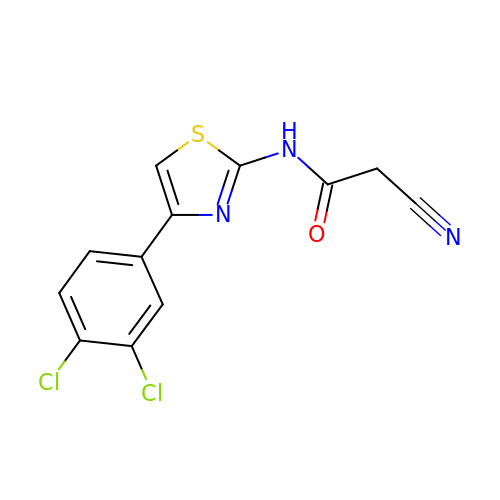2-cyano-~{N}-[4-(3,4-dichlorophenyl)-1,3-thiazol-2-yl]ethanamide | C12 H7 Cl2 N3 O S | UVZNRMKUEHJMJX-UHFFFAOYSA-N>[4x]MTYKGYLIDLDGTIYKGKDRIPAGEDFVKRLQERQLPYILVT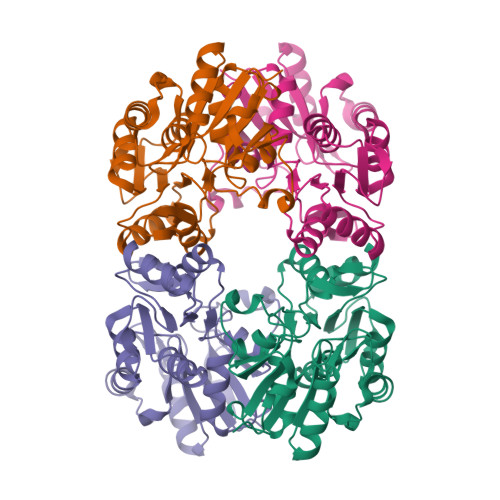NNTTRTPEMVQEMLATSFNIKTPLETIYTATLATIDYMNDMKRGKTAYVIGETGLKKAVAEAGYREDSENPAYVVVGLDTNLTYEKLTLATLAIQKGAVFIGTNPDLNIPTERGLLPGAGAILFLLEKATRVKPIIIGKPEAVIMNKALDRLGVKRHEAIMVGDNYLTDITAGIKNDIATLLVTTGFTKPEEVPALPIQPDFVLSSLAEWDFDER> G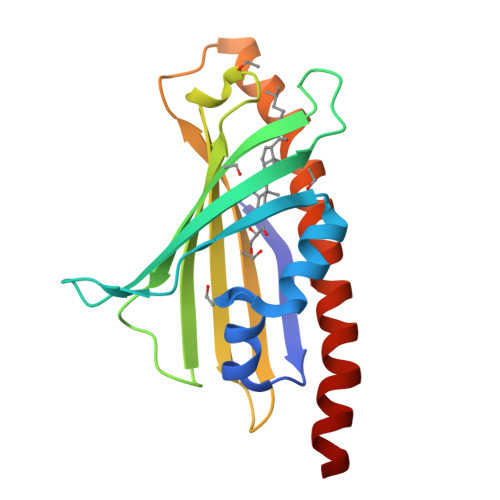RLYINRVFHISAERMFELLFTSSHFMQRFANSRNIIDVVSTPWTVESGGNQLRTMTYTIVLSNPLTGKYTAATEKQTLYKESREAQFYLVDSEVLTHDVPYHDYFYTLNRYCIVRSAKQRCRLRVSTDLKYRKQPWGLIKSLIEKNSWSSLESYFKKLESDLLMEESVLSQSIEDA>[4x]MATSGFSKPLHYPPVRRDETVVDDYFGVKVADPYRWLEDPNSEETKEFVDNQEKLANSVLEECELIDKFKQKIIDFVNFPRCGVPFRRANKYFHFYNSGLQAQNVFQMQDDLDGKPEVLYDPNLREGGRSGLSLYSVSEDAKYFAFGIHSGLTEWVTIKILKTEDRSYLPDTLEWVKFSPAIWTHDNKGFFYCPYPPLKEGEDHMTRSAVNQEARYHFLGTDQSEDILLWRDLENPAHHLKCQITDDGKYFLLYILDGCDDANKVYCLDLTKLPNGLESFRGREDSAPFMKLIDSFDASYTAIANDGSVFTFQTNKDAPRKKLVRVDLNNPSVWTDLVPESKKDLLESAHAVNENQLILRYLSDVKHVLEI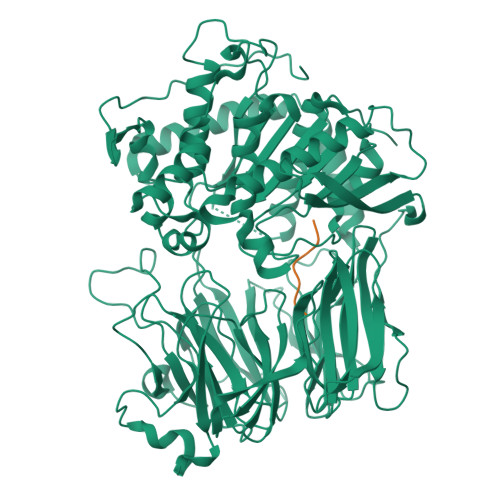RDLESGALQHRLPIDIGSVDGITARRRDSVVFFKFTSILTPGIVYQCDLKNDPTQLKIFRESVVPDFDRSEFEVKQVFVPSKDGTKIPIFIAARKGISLDGSHPCEMHGYGGFGINMMPTFSASRIVFLKHLGGVFCLANIRGGGEYGEEWHKAGFRDKKQNVFDDFISAAEYLISSGYTKARRVAIEGGANGGLLVAACINQRPDLFGCAEANCGVMDMLRFHKFTLGYLWTGDYGCSDKEEEFKWLIKYSPIHNVRRPWEQPGNEETQYPATMILTADHDDRVVPLHSFKLLATMQHVLCTSLEDSPQKNPIIARIQRKAAHYGRATMTQIAEVADRYGFMAKALEAPWID;>[4x]MSPILAHDVVKPQGVPVWAFQAKDVENASAPV> MRQLLLISDLDNTWVGDQQALEHLQEYLGDRRGNFYLAYATGRSYHSARELQKQVGLMEPDYWLTAVGSEIYHPEGLDQHWADYLSEHWQRDILQAIADGFEALKPQSPLEQNPWKISYHLDPQACPTVIDQLTEMLKETGIPVQVIFSSGKDVDLLPQRSNKGNATQYLQQHLAMEPSQTLVCGDSGNDIGLFETSARGVIVRNAQPELLHWYD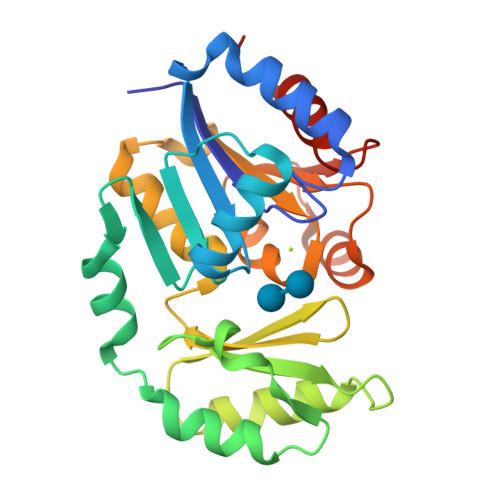QWGDSRHYRAQSSHAGAILEAIAHFDFLS>VFHKIRNEDLIFNESLGQGTFTKIFKGVRREVGDYGQLHETEVLLKVLDKAHRNYSESFFEAASMMSKL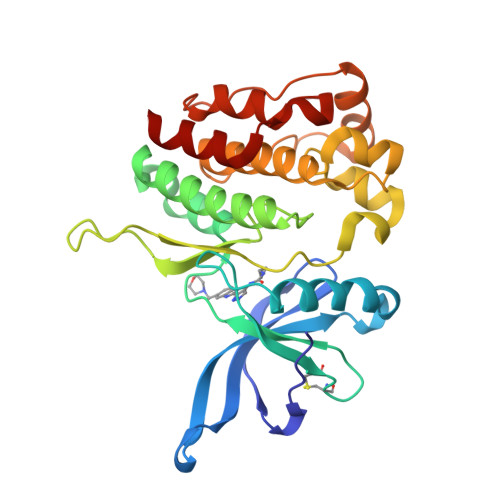SHKHLVLNYGVCFCGDENILVQEFVKFGSLDTYLKKNKNCINILWKLEVAKQLAAAMHFLEENTLIHGNVCAKNILLIREEDRKTGNPPFIKLSDPGISITVLPKDILQERIPWVPPECIENPKNLNLATDKWSFGTTLWEICSGGDKPLSALDSQRKLQFYEDRHQLPAPKAAELANLINNCMDYEPDHRPSFRAIIRDLNSL[2x]>GGGGGGMADLFSTVQEKVAGKDVKIVFPEGLDERILEAVSKLAGNKVLNPIVIGNENEIQAKAKELNL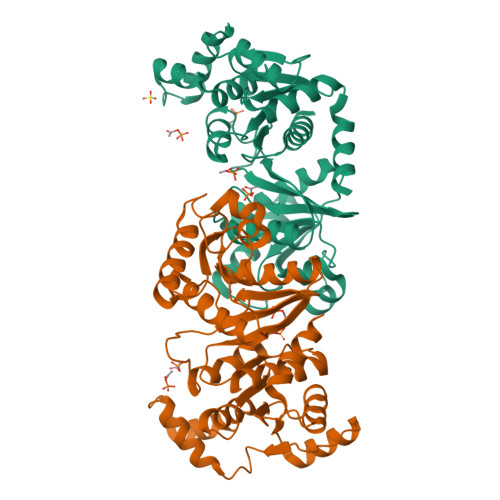TLGGVKIYDPHTYEGMEDLVQAFVERRKGKATEEQARKALLDENYFGTMLVYKGLADGLVSGAAHSTADTVRPALQIIKTKEGVKKTSGVFIMARGEEQYVFADCAINIAPDSQDLAEIAIESANTAKMFDIEPRVAMLSFSTKGSAKSDETEKVADAVKIAKEKAPELTLDGEFQFDAAFVPSVAEKKAPDSEIKGDANVFVFPSLEAGNIGYKIAQRLGNFEAVGPILQGLNMPVNDLSRGCNAEDVYNLALITAAQAL[6x]> MGSSHHHHHHSQDPQDLNFGQVVADVLCEFLEVAVHLILYVREVYPVGIFQKRKKYNVPVQ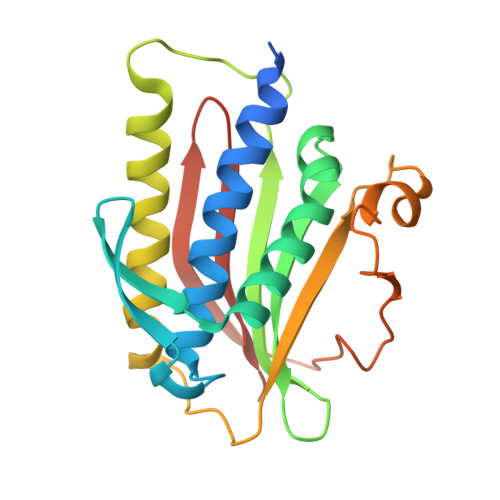MSCHPELNQYIQDTLHCVKPLLEKNDVEKVVVVILDKEHRPVEKFVFEITQPPLLSISSDSLLSHVEQLLAAFILKISVCDAVLDHNPPGCTFTVLVHTREAATRNMEKIQVIKDFPWILADEQDVHMHDPRLIPLKTMTSDILKMQLYVEERAHKGS>[4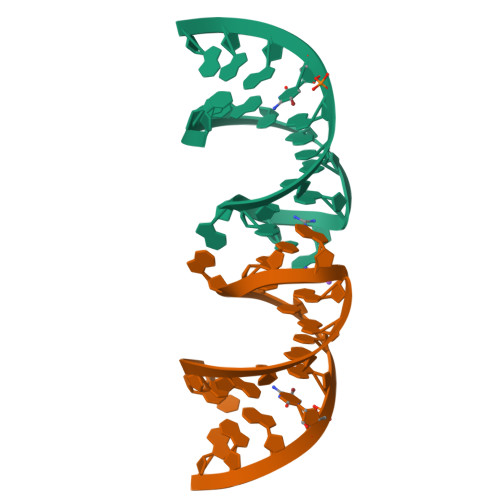x]UUUGCAGGACGACCUGCAAA>GSEELLDLFNRQVTQEFTASQVYLSASIWFDQNDWEGMAAYMLAQSAEEREHGLGFVDFANKRNIPIELQAVPAPVSCAEWSSPEDVWQSILELEQANTRSLLNLAEAASTCHDFAVMAFLNPFHLQQVNEEDKIGSILAKVTDENRTPGLLRSLDVVSFLGPCLFRSV[8x]

Ferritin from the marine pennate diatom Pseudo-nitzschia multiseries (PmFTN) plays a key role in sustaining growth in iron-limited ocean environments. Typically formed from 24 subunits arranged as a symmetric, hollow sphere, ferritins take up soluble Fe2+ and catalyze its oxidation, with the resulting Fe3+ being stored as an oxy-hydroxide mineral in its central cavity. The di-iron catalytic ferroxidase center of PmFTN (sites A and B) has a nearby third iron site (site C) in an arrangement typically observed in prokaryotic ferritins. Here we demonstrate that Glu-44, a site C ligand, and Glu-130, a residue that bridges iron bound at sites B and C, limit the rate of post-oxidation reorganization of iron coordination and the rate at which Fe3+ exits the ferroxidase center for storage within the mineral core.

Three crystal structures were obtained from E44Q PmFTN crystals soaked for 5 min (E44Q Fe (5 min)), 45 min (E44Q Fe (45 min)), and overnight (E44Q Fe (o.n.)) in an aerobic Fe2+ solution. Iron was observed bound at sites A and B with near full occupancy, whereas site C was empty. Residue Glu-47 was part of site C in wild type PmFTN; however, in the E44Q variant structure, the side chain of this residue is instead pointing into the mineral core, and in five of eight subunits within the asymmetric unit, up to two iron ions are observed to be coordinated to Glu-47. These iron ions were modeled at 25–35% occupancy and occupy distinct sites from those observed in wild type PmFTN. In E44Q Fe (o.n.), an additional iron ion was modeled within some of the B-channels. The iron ion is close to the inner surface, coordinated by Glu-35, weakly coordinated by Asp-30, and coordinated by up to two solvent molecules, and modeled with occupancies of 25–35%. Glu-35 adopts two conformations, one coordinating to the iron ion and one pointing away from the channel. The E44Q Fe (o.n.) structure provides evidence that these channels can accommodate iron, coordinated toward the cavity end of the channel by Glu-35, Asp-30, and up to two water molecules. Interestingly, iron ions at the B-channels were not observed in the wild type protein or in any of the other variants, suggesting that binding of iron in the B-channels is enhanced in the E44Q variant. However, structural data suggest that there is no change of iron location, as Fe-A and Fe-B are fully occupied in E44Q PmFTN following overnight iron soak.>[6x]ETGHHHHHHDDANVVRDRDLEVDTTLKSLSQQIENIRSPEGSRKNPARTCRDLKMCHSDWKSGEYWIDPNQGCNLDAIKVFCNMETGETCVYPTQPSVAQKNWYISKNPKDKRHVWFGESMTDGFQFEYGGQGSDPADVAIQLTFLRLMSTEASQQITYHCKNSVAYMDQQTGNLKKALLLQGSNEIEIRAEGNSRFTYSVTVDGCTSHTGAWGKTVIEYKTTKSSRLPIIDVAPLDVGAPDQEFGFDVGPVCFL

Fibrillar collagen molecules are synthesized in precursor form, procollagens, consisting of a rod-like central triple-helical region (∼300 kDa) with globular propeptide extensions at both the N- (∼50 kDa) and C- (∼90 kDa) termini. Though this collagen mostly occurs as a heterotrimer with two α1(I) chains and one α2(I) chain, small amounts of a homotrimeric form (three α1(I) chains) have been reported in adult skin as well as greater levels in embryonic tissues. Inside the cell, within the endoplasmic reticulum, the C-propeptides (also called COLFI domains) play key roles in determining correct chain association during trimerization, notably in cells producing different collagen types. While in general the amino acid sequences of the C-propeptides are highly conserved, Lees et al. identified a highly variable so-called chain recognition sequence (CRS) which appeared to be required for specific chain recognition during trimer assembly.

Here we present the crystal structure of the homotrimeric form of CPI (homo-CPI) determined to 2.2 Å resolution which shows striking differences in the inter-chain interface compared to CPIII. The overall structure of the homo-CPI trimer strongly resembles that of CPIII having the shape of a flower, with a stalk, a base and three petals. There are two trimers in the asymmetric unit, the structures of which are very similar (root mean square deviation (r.m.s.d.)=0.67 Å), with only slight movements in the stalk and petal regions. The stalk consists of an α-helical three-stranded coiled-coil formed by residues 8–29. Residues 30–76 form the base region, which is particularly highly conserved among the different fibrillar procollagens. This region includes three tightly bound Ca2+ ions (one per chain; same coordination as in CPIII) and one Cl− ion in the centre coordinated by Gln62 and Arg39 from all three chains, as well as one intra-chain (Cys41–Cys73) and one inter-chain (Cys47–Cys64) disulfide bond. The remainder of the molecule constitutes the petal region (residues 77–246) which is stabilized by two intra-chain disulfide bonds (Cys81–Cys244, Cys152–Cys197) and contains the long and short stretches of the CRS. The main difference is in the orientation of helix-4, a relatively long α-helix in each chain whose ends are involved in the inter-chain interactions thus forming a central triangle in the trimer. While the inter-chain interface in CPIII is characterized by a relatively large number of specific interactions (salt bridges and hydrogen bonds) involving residues in the CRS28, there are surprisingly few of these interactions in homo-CPI. The only example involving the CRS is the salt bridge between Asp129 (CRS long) and the highly conserved Arg42 situated in helix-2 in the base region. Instead, homo-CPI seems to be stabilized by interactions mainly involving residues in the base region.1-ISOBUTOXY-2-PYRROLIDINO-3[N-BENZYLANILINO] 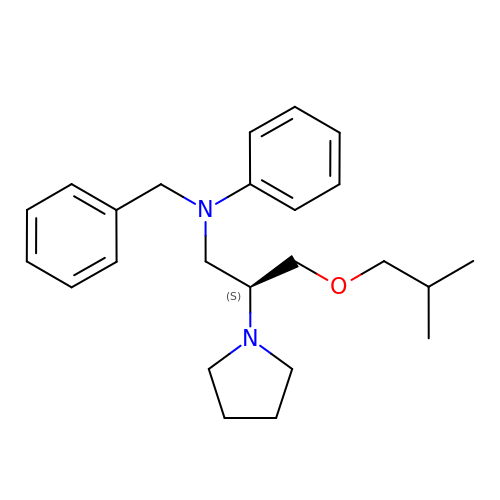PROPANE | C24 H34 N2 O | UIEATEWHFDRYRU-DEOSSOPVSA-N> GSHGYVTVKPRVRL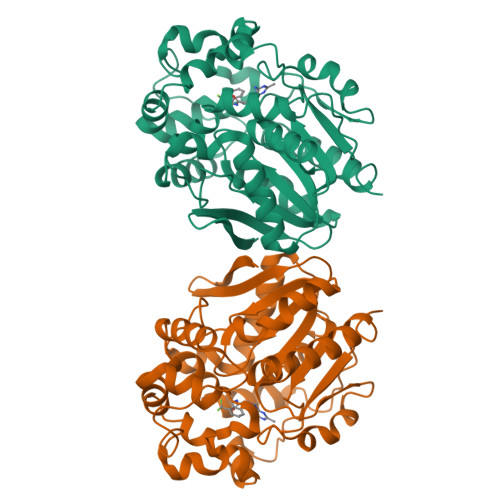HFVELGSGPAVCLCHGFPESWYSWRYQIPALAQAGYRVLAMDMKGYGESSAPPEIEEYCMEVLCKEMVTFLDKLGLSQAVFIGHDWGGMLVWYMALFYPERVRAVASLNTPFIPANPNMSPLESIKANPVFDYQLYFQEPGVAEAELEQNLSRTFKSLFRASDESVLSMHKVCEAGGLFVNSPEEPSLSRMVTEEEIQFYVQQFKKSGFRGPLNWYRNMERNWKWACKSLGRKILIPALMVTAEKDFVLVPQMSQHMEDWIPHLKRGHIEDCGHWTQMDKPTEVNQILIKWLDSDARNPAD>MWITQEITPYLRKEYTIEAKLLDVRSEHNILEIFKSKDFGEIAMLNRQLLFKNFLHIESELLAHMGGCTKKELKEVLIVDGFDLELAHQLFKYDTHIDFVQADEKILDSFISFFPHFHEVKNNKNFTHAKQLLDLDIKKYDLIFCLQEPDIHRIDGLKRMLKEDGVFISVAKHPLLEHVSMQNALKNMGGVFSVAMPFVAPLRILSNKGYIYASFKTHPLKDLMTPKIEALTSVRYYNEDIHRAAFALPKNLQEVFK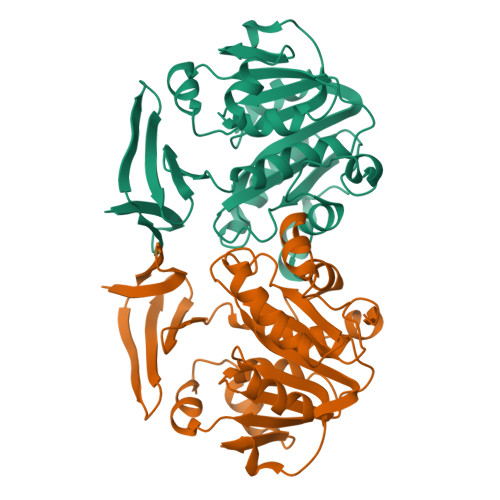DNIKS[2x]>MSLAQGRQVIGLDIGTTSTIAILVRLPDTVVAVASRPTTLSSPHPGWAEEDPAQWWDNARAVLAELKTTAGESDWRPGGICVTGMLPAVVLLDDRGAVLRPSIQQSDGRCGDEVAELRAEVDSEAFLARTGNGVTQQLVTAKLRWIERHEPAVFGAIATVCGSYDYINMLLTGERVVDRNWALEGGFIDLASGTVEADLVALAHIPPSAVPPAHPTHRVLGAVTAEAAALTGLPTGLPVYGGAADHIASALAAGITRPGDVLLKFGGAGDIIVASATAKSDPRLYLDYHLVPGLYAPNGCMAATGSALNWLAKLLAPEAGEAAHAQLDALAAEVPAGADGLV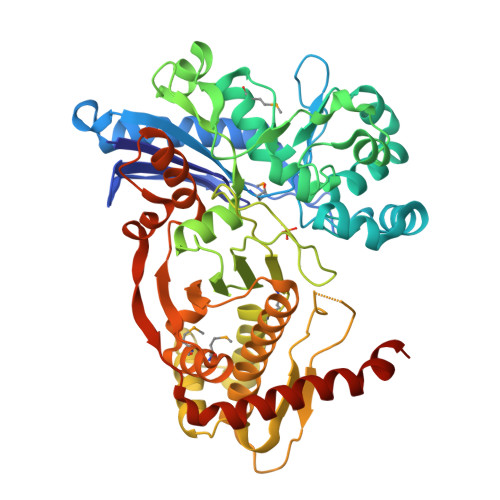CLPYFLGEKTPIHDPFASGTFTGLSLSHTRGHLWRALLEAVALAFRHHVAVLDDIGHAPQRFFASDGGTRSRVWMGIMADVLQRPVQLLANPLGSAVGAAWVAAIGGGDDLGWDDVTALVRTGEKITPDPAKAEVYDRLYRDFSALYATLHPFFHRSREGHHHHHH[2x]>[2x]GSGGSGKVVKFSYMWTINNFSFCREEMGEVIKSSTFSSGANDKLKWCLRVNPKGLDEESKDYLSLYLLLVSCPKSEVRAKFKFSILNAKGEETKAMESQRAYRFVQGKDWGFKKFIR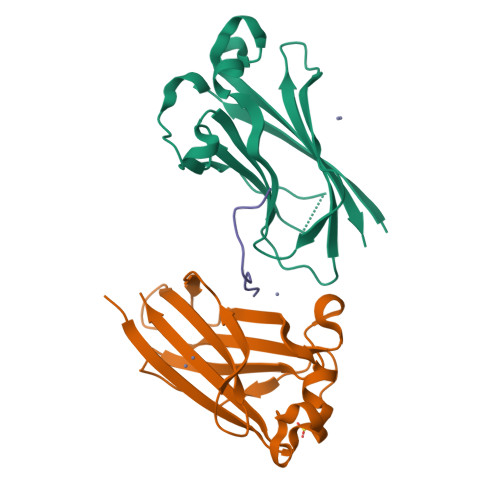RGFLLDEANGLLPDDKLTLFCEVSVVQD;> XDSTTEGTPADGFTVL> RIHNRMLRARILKLDGKDYRPEEQAAFDLLRDGLLDGISNRKSTPKLDVYSDQIVWGRSPVRIDMAGGWTDTPPYSLYSGGNVVNLAIELNGQPPLQVYVKPCKDFHIVLRSIDMGAMEIVSTFDELQDYKKIGSPFSIPKAALSLAGFAPAFSAVSYASLEEQLKDFGAGIEVTLLAAIPAGSGLGTSSILASTVLGAINDF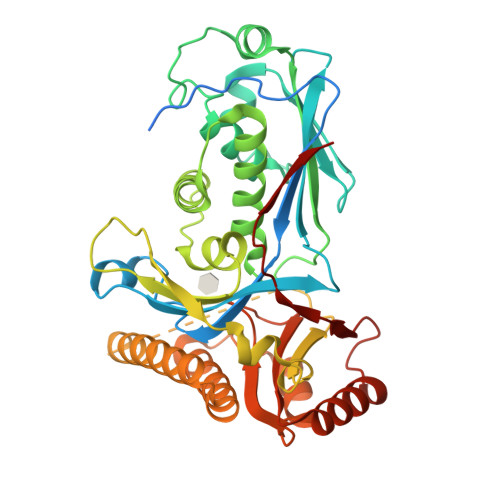CGLAWDKNEICQRTLVLEQLLTTGGGWQDQYGGVLQGVKLLQTEAGFAQSPLVRWLPDHLFTHPEYKDCHLLYYTGITRTAKGILAEIVSSMFLNSSLHLNLLSEMKAHALDMNEAIQRGSFVEFGRLVGKTWEQNKALDSGTNPPAVEAIIDLIKDYTLGYKLPGAGGGGYLYMVAKDPQAAVRIRKILTENAPNPRARFVEMTLSDKGFQVSRS> SMQGNWNMGPPGGLQEFNFIVPTGKTGLIIGKGGETIKSISQQSGARIELQRNPPPNADPNMKLFTIRGTPQQIDYARQLIEEKIGGPVNPLG

Far upstream element (FUSE) binding protein 1 (FUBP1 or FBP1) is a multifunctional single-stranded DNA- (ssDNA) and RNA-binding protein, which acts as a master regulator of diverse cellular processes including transcription, mRNA stability and translation as well as RNA splicing. Central to its single-stranded nucleic acid (ssNA) interacting function of human FUBP1 is a tandem of four K homology (KH) motifs, namely KH1, KH2, KH3 and KH4, which is embedded in the middle region in between the self-regulatory and transactivation domains at the N- and C- termini, respectively. Comparison of the four structures showed that they all adopted an evolutionarily conserved eukaryotic KH-domain architecture, consisting of a three-stranded β-sheet packed on one side by three helices. A common property in recognition of up to four nucleotides is facilitated by a ‘minimal KH motif’ that constructs an ssNA hydrophobic binding cleft formed on one side by two short consecutive helices (α1 and α2) and the GXXG-motif-containing connecting loop and on the other side by the domain’s β-sheet and the variable loop that links the β2 and β3.

In contrast to the upper part of the binding pocket, considerable variations of the amino acid compositions within α1 and the β2-β3 connecting loop led to the remarkably distinct properties of the nucleotide binding pocket at the lower half, which is responsible for interacting with ssDNA nucleobases. For instance, a longer loop together with the presence of small hydrophobic (A194 and A197) or polar residues (T385 and T388) in α1 of KH2 and 4, respectively, resulted in relatively open binding surface with strong positively-charged electrostatic potentials. In contrast, the migration patterns of KH2 and KH4 were rather ambiguous with some slight shifts observed for nearly all nucleotides, except fragment 4 and 10 that had a high GC-rich content. Interestingly, the potential interactions of KH2 and 4 with ssDNA 5–8, which shared the presence of a triple-repeated deoxythymidine (TTT), was consistent with the previous suggestion on the preference of FUBP1 for T-enriched sequence. In addition, we observed interestingly also that KH2 preferred the T-rich fragment 7 over the TGTG-core fragment 8, which was in contrast to KH4 that showed no preference for both ssDNA. As expected, in contrast to the wild type, all mutants did not show a shift in migration on native gels upon incubation with the selected ssDNA. These overall results suggested therefore that all four KH motifs of FUBP1 interacted with c-Myc FUSE ssDNA independently and individually, and KH1 and 3 might exert potential preference for ‘TTTGTGTT’ sequence while KH2 and KH4 might have broader binding specificity.> MQTPSIIQCGLLNSFARKMTDAISDNQIIATSRFFNIARDVADVVVSNTKLAQQYEQLSIDSLKEYLVSVAKFVAVDYSNTTSADVDDLIHKLRLFIEEECYQYNIDKEETCDGDVCVSDEYNEPAPKPKPKPKPKPAPKPKPAPKPKPAPKPAPKPAPKPAPKPAPKPAPKPAPKPAPEPAPEPAPEPAPKPAPEPAPEPAPIRPARRCDENPSNLETCCTNKALYGDFTDSSCDIVKKKTNWWLWGGIAILVIVLMIGGYFIYKRYFSAPKFENTGEFVNDMNFNNDVNFNNDVNFDNDMNYGNEGIDVSDLEILNLPVPSVSPVPSASIVPSVSPIPRGSPVPSASPIK;> MKTETLYQDPVWFQDLSVIFKRPSEIIPTRDQSDSERINAMVRLVLYCSFAVALIRQNYLYAILGLAIIAIISLAYALGAKKTKSNEAYGNIRPYSVKRSKKSCSKSSANNPFSNATVGALLDNEARPPACSYDDNDMASTMRKNFNKGLFRNLDDVYEVENSQRQFYTMPVTTAAPDLTAFGQFLYGSKGKTCKEDPSACTPAFATRDG;>MMNFILVLLIVAMIGTILVSESKYLFSKPVCKNCGVKAVTLPVDISAGKLAKVAEAVKKQTEEIKTLLKQKQSAPKAPELTNPIEHIKASTTVVSGANGLENVIDEDLPFSDFKGVPVAETTVEGMIKGIRPPTYADPRVMNPALAAAPVQFSDPTQFGTFGVTDDVSPAFSTEDKIPKTNAKISSDISVEGYENSYDANGARLVMDGKVVKSECQLPSYQIRNSKHHTQLPMRSLNEPPPMVEDLVDESLFEGLQGYPVDEKLDLLTPPGTATPSSEWAAINYGLTNN[2x];> MQIYSEYYEKIGPRKLRLLVKRRLLFASTWLYINNYILLSIIMKLQTKHMILLGFVAVVVVFIIFMLTRKKKEGFSIGNIFGKVKGAVTGTVGKVVNVVKPQGYKPEFVNRVNFGKFWACPEGTTDWGSEDKQCLVSQYGPMMWRNKGGNEWGWSCPAGSAPNNSDDWNQKCVQGYSMKKLIDGQWRCTDTEIDTGKDWSNSDWFTAQQQCDRGNNKVFTRRMYIDGKWQCPDGTWDTGFTWSDGENGGKQCKYYP;> MILVGIAVLILLAVFAILYYKQKEKFVVVGKFVEPIPSNPGQDFTLLPMDQTYTFADPVPDTATAFDVVLSRFTDKKAPADLLKGATFPEAAPYTDSEVENISKLALSRVKGPDAPVLSFISVEYAAKGVDNKKNTHYDIAFMVYDQVKNFSLKLVLVAVLDAKNKLWIKKFSSFNSFTPKDKGPKGVENIDETPLAEFIPDFVQFSRLYKDNANV;> MVETTQHFVSIESSNRPDPANTTPANYSIQLPQRYRNIWSAMLVNIALPAVSPPQKYVYLDIDKLNSIDSTSPSGGVNFALAKIPLSIAGTGNVFFADTMTSSFPNVPLQNPVATMDKLNIKLKDANGNVLTIPAGNEHSFMIQLTCGDYIPRGGGSTITQNGRVLGGTR;> MGNGPPMERAVSSDDILTYYNTFIFFIYFNFTNENIYIIYTIYMKVQNTIVYIVLLLIVVVIIWNFTRKEGWSDYNAPNDFMKIYYSNIVEDKKLAEKYPFFGTGPFTGLRCRKPNNVGCNTTWVSGQLVELTPKLKEQIECKFGIQYVKT;> MDSRLSAAYAIRAARISMIPGGVDGLVINYAEGGEPAWVQYPLKKQKPLPNNLCYTPTLEDIARKREAVIAKYTKQPLETGTTFTHVLNASHLNEQYTRVKKSALPDKEFPIIETEKYPEPPILWETTIGAPSRLFDRSDGVKYVR;>[12x]MDMHMIVKVVAILAVLFLVYKLWESMNKPNASPLKIQNPYEKYMNSAEGGEYDAEDDDIYYPETDAEDDDIYTGETDDMYDGEDDDIYVQEGDDIEDAEDEPYDDSADMEQDVPKVQQPMMPLLTPSSQLLPKPSPEAADFAQFAPKNLQAQNFLTATQWIGVNTQGSSLKNANYDLRADPIIPKADVGPWMMSSVDPNIYQKPLFG;> MCNTYYKRVKFNLFLYTNSIEMELLAVASIIGYGLFSSQQGRETRPDRNRYAEALGSGQGLDEDYDVKPTDMVRKYRKKAEKRWKKAQVPKESGIITPNMRPSEVMPYFTSGKSMNTNTDYKQRKMELFTGGVLDGHSVSGTYKHKVEAANMFGMTPQGRVTSDGTVGNAPGDTELLKARSVNSHQYNNVLPTEQLRVGPGLGVGPEVAATGGFHQFYRQLPLNINEYKLTQLPGRLVPGGTTTGGKGEIQQIASVNHNPDALVLNYDDRPPEATPNGAILASTQYGKQPRGYAGLRPYEKNYEGIAEADVSALQARYLDQTRGRPRTGDGDTEPIINPNGERDGTGSYVTENMCSMTLESQRGLVNRYITPPGVTGVVQQGGEMRPEFVPETTIREQYEDIYYTGPAGTTVTPTEPMNVVELQPESRHAKRAGQDRAYTPGAGRVNNFAPAAQGAYGLKDHPTYNALQHVVSEPIEQTFLPAAQGDDDRFGTKSNVNNPWGNPASLQIANNQLAANKFNRDVTNTVNLDYDAGQPMKQQNFQPKAWIPNNTDDMKMLPLWKRKQLQAQKNKQQRK;>MFSAFRDTASIGFSDTHQDEKTLRFLKKQISQFIKHLKEYYPNNELTKKLVMKYSDVQLLPYTKGATKDTYTSGLFDHTTGVIKIAPRDGLGNVRDEQSLNKSICHELAHGTRVKYPGESSHSDEWKDAWKTFLKIAADELGWKIEVPCSSVSFYGLTKDDCENCVWDQDPETCPKTAKLA[4x];>[3x]MAMKTQRKENVLFQNVKPREIPLVDNPFSTYPYKHVITETQPTQAKNQAIWGLVQMGLSGEAAAMYGDVVVQKTTRACRKSEGGFKDVNTELWGTSPYLGRGDGEVYNMPASNQLLRGFESSLRGSRVRTQIDDKSFIPYTWQMIDVPLAAAKTSFIAGLDTRQQLAYGNP;> METIGNFIQNMAFPTENPYKLSGDFGNSTLEPTVTAALRILHESPAPFNTEFFSRKNVDFIQKKLISETKRYTSFDIGPQNEDELIMMMAGIYVQDSTFDGNIKAGLRKLNTLVITECLKQILPGVRAYALYVRDASLPFSGGGEEAFKRPELATLKGSKVLSGFLPLDRNAS;>MAGGLSQLVAYGAQDVYLTGNPQITFFKTVYRRYTNFAIESIQQTINGSVGFGNKVSTQISRNGDLITDIVVEFVLTKGGNGGTTYYPAEELLQDVELEIGGQRIDKHYNDWFRTYDALFRMNDDRYNYRRMTDWVNNELVGAQKRFYVPLIFFFNQTPGLALPLIALQYHEVKLYFTLASQVQGVNYNGSSAIAGAAQPTMSVWVDYIFLDTQERTRFAQLPHEYLIEQLQFTGSETATPSATTQASQNIRLNFNHPTKYLAWNFNNPTNYGQYTALANIPGACSGAGTAAATVTTPDYGNTGTYNEQLAVLDSAKIQLNGQDRFATRKGSYFNKVQPYQSIGGVTPAGVYLYSFALKPAGRQPSGTCNFSRIDNATLSLTYKTCSIDATSPAAVLGNTETVTANTATLLTALNIYAKNYNVLRIMSGMGGLAYAN[84x];> MHKITPFLIAAVVAVIVLAVWLFKKDNKKETWFSRDLNYGKANSKIWNATVAKGLKGIANENAEIRKMYPYLGYGDFTGAICKGPNNQGCTYYANYTR

The PBCV-1 nucleocapsid is enclosed by a lipid bilayer membrane. The membrane is surrounded by a roughly icosahedral external capsid shell that has a unique vertex where a spike structure, required for host entry, is located. The outer capsid shell of the icosahedrally averaged PBCV-1 structure consists of the MCP (Vp54) and the penton protein. The minor capsid proteins (P2, P3, P4, P5, P6, P7, P8, P9, P10, P11, P12, P13, and P14) form a hexagonal network that is immediately below (inside) the outer capsid shell.

Here we have extended the resolution of the PBCV-1 structure to 3.5 Å by collecting data using a direct electron detector. The improved resolution of the cryo-EM map resulted in the identification of 13 different minor capsid proteins and an atomic model of the viral capsid consisting of 6900 polypeptide chains. This is by far the largest viral capsid structure that has been determined to near-atomic resolution, and the first near-atomic description of a NCLDV capsid. Each icosahedral asymmetric unit of the outer capsid shell contains 28 pseudo-hexameric capsomers with 6 of these in the pentasymmetron (a, b, c, d, e, and f) and 22 in the trisymmetron (A, B, C, D, E, F, G, H, I, J, K, L, M, N, O, P, Q, R, S, T, U, and V). P2, P5, P6, P7, P8, P9, P12, P13, and P14 are present as a single copy in each icosahedral asymmetric unit, whereas the copy number per icosahedral asymmetric unit of P3, P4, P10, and P11 are three, four, two and 12, respectively. Three rows of P3 and three copies of P2 construct a scaffold that glues together all the capsomers in each trisymmetron. The N terminus of each P2 protein extends to a neighboring pentasymmetron and glues together one-fifth of the pseudo-hexameric capsomers in a pentasymmetron. Neighboring symmetrons are bound together by the zip proteins (P11). P2 essentially acts as a molecular tape measure (or ruler) and determines the size of the viral capsid. The icosahedrally averaged near-atomic structure of PBCV-1 shows that the PBCV-1 capsid is stabilized by a dense array of minor capsid proteins (P2–P14) inside the major capsid shell. This minor capsid protein shell cements most of the gaps between neighboring capsomers and uses transmembrane helices to mediate inner viral membrane association.4-[4-[3-[5-[(3~{S})-4,4-dimethyl-3-oxidanyl-pentyl]-4-methyl-1,3-thiazol-2-yl]pentan-3-yl]phenoxy]-~{N}-oxidanyl-butanamide | C26 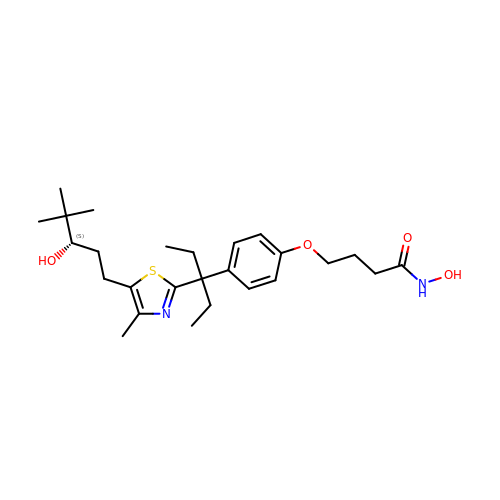H40 N2 O4 S | CHEHAHOVAVDOHQ-QFIPXVFZSA-N> MERTELLKPRTLADLIRILHELFAGDEVNV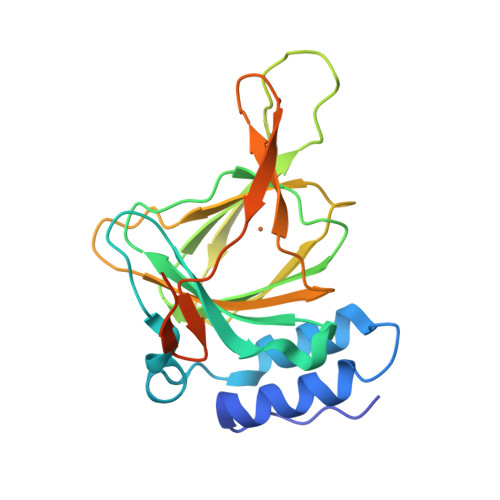EEVQAVLEAYESNPAEWALYAKFDQYRYTRNLVDQGNGKFNLMILCWGEGHGSSIHDHTDSHCFLKLLQGNLKETLFDWPDKKSNEMIKKSERTLRENQCAYINDSIGLHRVENVSHTEPAVSLQLYSPPFDTCHAFDQRTGHKNKVTMTFHSKFGIRTPFTTSGSLENNSAWSHPQFEK(2R)-2-cyano-3-[3-(1H-pyrrolo[2,3-b]pyridin-3-ylcarbonyl)phenyl]propanamide | C18 H14 N4 O2 | 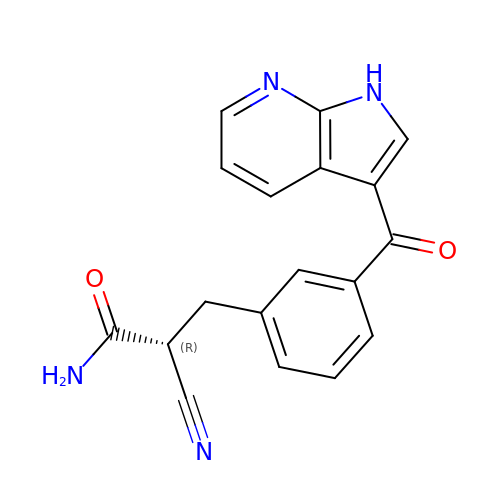UQJDULLQUOPWND-CYBMUJFWSA-N Sterile alpha motif and HD domain-containing protein 1 (SAMHD1) is an important regulator of cellular 2′-deoxynucleoside-5′-triphosphate (dNTP) in mammalian cells. Although the HD-domain contains the active site, dNTP hydrolysis requires assembly of SAMHD1 into homo-tetramers. Here, sequences at the N and C termini of the HD-domain stabilise inter-monomer protein–protein interactions and incorporate four pairs of allosteric nucleotide-binding sites, AL1 and AL2, which regulate the enzyme through combined binding of G-based (AL1) and 2′-deoxynucleoside (AL2) triphosphates. Using combined biophysical and X-ray structural studies incorporating nucleotide analogues along with mutagenesis experiments we have now discovered that SAMHD1 uses a bi-metallic Fe–Mg centre to catalyse dNTP hydrolysis in a reaction similar to those catalysed by HD domains in both human and bacterial phosphodiesterase PDE enzymes.

Co-crystal structures were determined using either wild-type (wt) wt-SAMHD1(109-626) or a D137N-SAMHD1(109-626) AL1 allosteric site mutant that generally produced higher resolution diffraction than wt co-crystals. A further effect of the D137N substitution is that D137N-SAMHD1 is activated by xanthosine-5′-triphosphate (XTP) rather than GTP through AL1-binding but nevertheless maintains comparable catalytic parameters for dNTP hydrolysis as those observed for wt-SAMHD1 and GTP. We first determined structures of two co-complexes of D137N-SAMHD1(109-626) in the presence of Mg2+, which is required for tetramer assembly and catalysis, with (i) XTP (AL1) and dAMPNPP (AL2 and active site), and (ii) XTP (AL1) and dGMPNPP (AL2 and active site). SEC-MALLS analysis revealed that all four dNMPNPP analogues, which have an imido substitution at the α,β-bridging oxygen, when combined with GTP, support the formation of stable SAMHD1 tetramers, albeit to varying degrees. Near-complete tetramerisation was observed with dAMPNPP, while dCMPNPP promoted the least tetramerisation and dGMPNPP was able to support tetramerisation without additional GTP, presumably by occupying both AL1 and AL2 allosteric sites. Further investigation using inhibition assays revealed that all dNMPNPP analogues were actually competitive inhibitors of SAMHD1-dNTP triphosphohydrolase activity, with inhibition constants (Ki) ranging from 0.78 µM for dAMPNPP to 0.052 µM for dGMPNPP, with the following rank order of increasing affinity: dAMPNPP < TMPNPP < dCMPNPP < dGMPNPP. The resolution of these structures varied between 2.0 and 3.2 Å, but all structures contain highly homologous “closed” tetramers of the SAMHD1 catalytic domain, with pairwise root-mean-square deviations (RMSDs) of <0.5 Å across all atoms in each tetramer.

>GSQIHVDTMKVINDPIHGHIELHPLLVRIINTPQFQRLRYIKQLGGGYYVFPGASHNRFEHSLGVGYLAGCLVHALGEKQPELQISERDVLCVQIAGLCHDLGHGPFSHMFDGRFIPLARPEVKWTHEQGSVMMFEHLINSNGIKPVMEQYGLIPEEDICFIKEQIVGPLESPVEDSLWPYKGRPENKSFLYEIVSNKRNGIDVDKWDYFARDCHHLGIQNNFDYKRFIKFARVCEVDNELRICARDKEVGNLYDMFHTRNSLHRRAYQHKVGNIIDTMITDAFLKADDYIEITGAGGKKYRISTAIDDMEAYTKLTDNIFLEILYSTDPKLKDAREILKQIEYRNLFKYVGETQPTGQIKIKREDYESLPKEVASAKPKVLLDVKLKAEDFIVDVINMDYGMQEKNPIDHVSFYCKTAPNRAIRITKNQVSQLLPEKFAEQLIRVYCKKVDRKSLYAARQYFVQWCADRNFTKPQDGDVIAPLITPQKKEWNDSTSVQNPTRLREASKSRVQLFKDDPM[16x]>[2x]GLPVCGETCVGGTCNTPGCTCS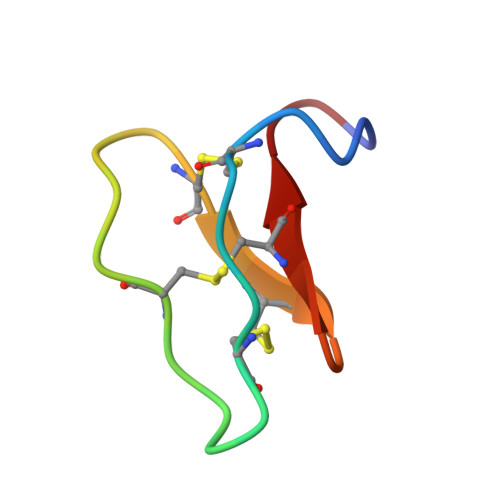WPVCTRN> MPFVNKQFNYKDPVNGVDIAYIKIPNAGQMQPVKAFKIHNKIWVIPERDTFTNPEEGDLNPPPEAKQVPVSYYDSTYLSTDNEKDNYLKGVTKLFERIYSTDLGRMLLTSIVRGIPFWGGSTIDTELKVIDTNCINVIQPDGSYRSEELNLVIIGPSADIIQFECKSFGHEVLNLTRNGYGSTQYIRFSPDFTFGFEESLEVDTNPLL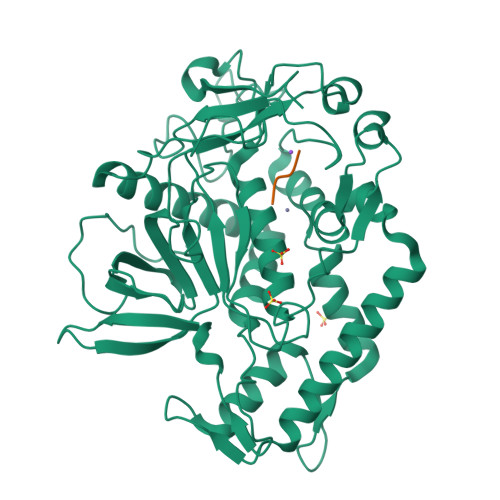GAGKFATDPAVTLAHELIHAGHRLYGIAINPNRVFKVNTNAYYEMSGLEVSFEELRTFGGHDAKFIDSLQENEFRLYYYNKFKDIASTLNKAKSIVGTTASLQYMKNVFKEKYLLSEDTSGKFSVDKLKFDKLYKMLTEIYTEDNFVKFFKVLNRKTYLNFDKAVFKINIVPKVNYTIYDGFNLRNTNLAANFNGQNTEINNMNFTKLKNFTGLFEHHHHHH;> RYGCX> DYVCGPLQRLKVKRQWAEAYGSGNSREEFGHFIWSHVFQHSPAARDMFKRVRGDNIHTPAF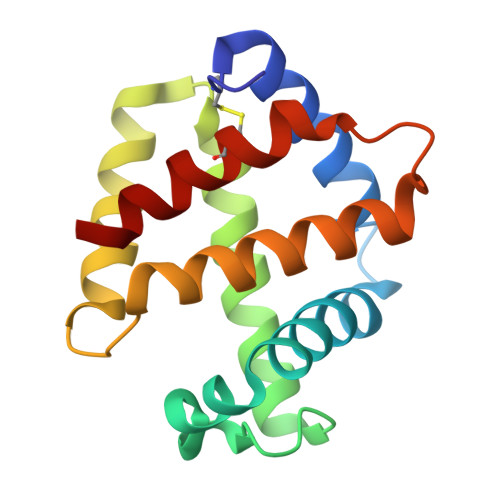RAHATRVLGGLDMCIALLDDEPVLNTQLAHLAKQHETRGVEAAHYDTVNHAVMMGVENVIGSEVFDQDAWKPCLNVITNGIQG6-(3,5-dimethoxyphenyl)-2-(4-methoxyphenyl)imidazo[1,2-a]pyridine | C22 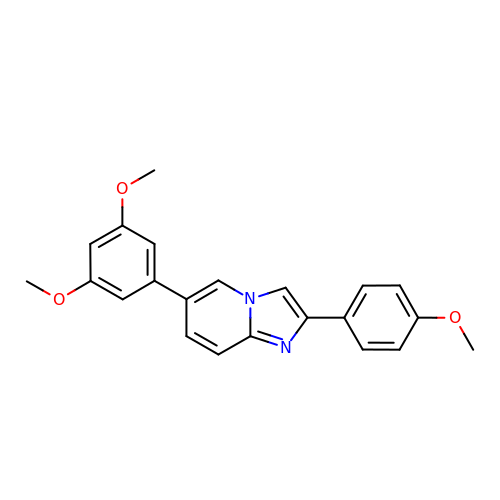H20 N2 O3 | IHJONSSVOHRQHD-UHFFFAOYSA-N>GSGHWGAWMPSTISAFEGTCVSIPCRFDFPDELRPAVVHGVWYFNSPYPKNYPPVVFKSRTQVVHESFQGRSRLLGDLGLRNCTLLLSTLSPELGGKYYFRGDLGGYNQYTFSEHSVLDIVNTPNIVVPPEVVAGTEVEVSCMVPDNCPELRPELSWLGHEGLGEPTV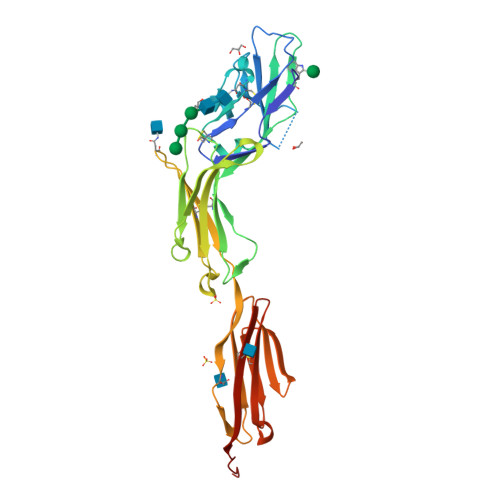LGRLREDEGTWVQVSLLHFVPTREANGHRLGCQAAFPNTTLQFEGYASLDVKYPPVIVEMNSSVEAIEGSHVSLLCGADSNPPPLLTWMRDGMVLREAVAKSLYLDLEEVTPGEDGVYACLAENAYGQDNRTVELSVMYAAAAHHHHHH[2x]>[3x]MKVLRHGLFKDRRVFDENYIPPELRVRRGEAEALARIYLNRLLSGAGLSDVNMIYGSIGRVGIGKTTLAKFTVKRVSEAAAKEGLTVKQAYVNA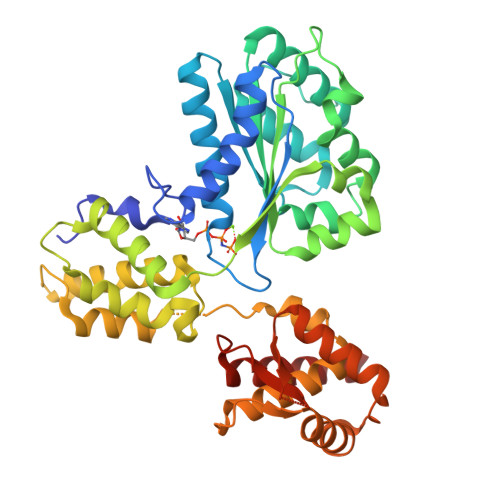FNAPNLYTILSLIVRQTGYPIQVRGAPALDILKALVDNLYVENHYLLVILDEFQSMLSSPRIAAEDLYTLLRVHEEIPSRDGVNRIGFLLVASDVRALSYMREKIPQVESQIGFKLHLPAYKSRELYTILEQRAELGLRDTVWEPRHLELISDVYGEDKGGDGSARRAIVALKMACEMAEAMGRDSLSEDLVRKAVSENEAASIQTHELEALSIHELIILRLIAEATLGGMEWINAGLLRQRYEDASLTMYNVKPRGYTQYHIYLKHLTSLGLVDAKPSGRGMRGRTTLFRLAPHLPADRLIEVVDNIIQAKMASGYE>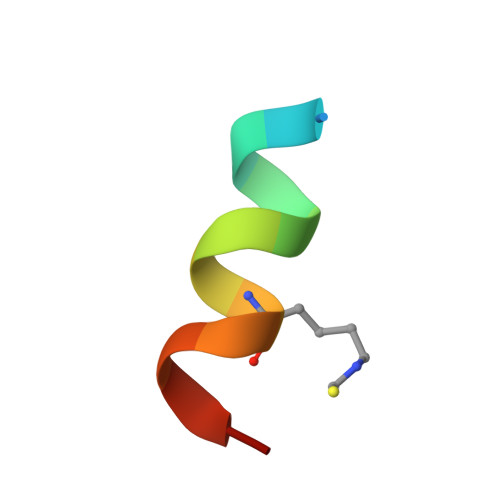 XTSFAEYWKLLSCX>[4x]APSRKFFVGGNWKMNGRKKNLGELITTLNAAKVPADTEVVCAPPTAYIDFARQKLDPKIAVAAQNCYKVTNGAFTGEISPGMIKDCGATWVVLGHSERRHVF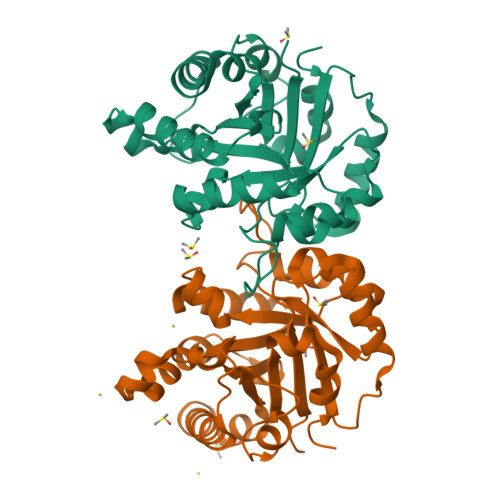GESDELIGQKVAHALSEGLGVIACIGEKLDEREAGITEKVVFEQTKVIADNVKDWSKVVLAYEPVWAIGTGKTATPQQAQEVHEKLRGWLKSNVSDAVAQSTRIIYGGSVTGATCKELASQPDVDGFLVGGASLKPEFVDIINAKQ> MVNISDFFGKNKKSVRSSTSRPTRQVGSSKPEVIDLDTESDQESTNKTPKKMPVSNVIDVSETPEGEKKLPLPAKRKASSPTVKPASSKKTKPSSKSSDSASNITAQDVLDKIPSLDLSNVHVKENAKFDFKSANSNADPDEIVSEIGSFPEGKPNCLLGLTIVFTGVLPTLERGASEALAKRYGARVTKSISSKTSVVVLGDEAGPKKLEKIKQLKIKAIDEEGFKQLIAGMPAEGGDGEAAEKARRKLEEQHNIATKEAELLVKKEEERSKKLAATRVSGGHLERDNVREEDKLWTVKYAPTNLQQVCGNKGSVMKLKNWLANWENSKKNSFKHAGKDGSGVFRAAMLYGPPGIGKTTAAHLVAQELGYDILEQNASDVRSKTLLNAGVKNALDNMSVVGYFKHNEEAQNLNGKHFVIIMDEVDGMSGGDRGGVGQLAQFCRKTSTPLILICNERNLPKMRPFDRVCLDIQFRRPDANSIKSRLMTIAIREKFKLDPNVIDRLIQTTRGDIRQVINLLSTISTTTKTINHENINEISKAWEKNIALKPFDIAHKMLDGQIYSDIGSRNFTLNDKIALYFDDFDFTPLMIQENYLSTRPSVLKPGQSHLEAVAEAANCISLGDIVEKKIRSSEQLWSLLPLHAVLSSVYPASKVAGHMAGRINFTAWLGQNSKSAKYYRLLQEIHYHTRLGTSTDKIGLRLDYLPTFRKRLLDPFLKQGADAISSVIEVMDDYYLTKEDWDSIMEFFVGPDVTTAIIKKIPATVKSGFTRKYNSMTHPVAIYRTGSTIGGGGVGTSTSTPDFEDVVDADDNPVPADDEETQDSSTDLKKDKLIKQKAKPTKRKTATSKPGGSKKRKTKA;> MSKTLSLQLPWVEKYRPQVLSDIVGNKETIDRLQQIAKDGNMPHMIISGMPGIGKTTSVHCLAHELLGRSYADGVLELNASDDRGIDVVRNQIKHFAQKKLHLPPGKHKIVILDEADSMTAGAQQALRRTMELYSNSTRFAFACNQSNKIIEPLQSRCAILRYSKLSDEDVLKRLLQIIKLEDVKYTNDGLEAIIFTAEGDMRQAINNLQSTVAGHGLVNADNVFKIVDSPHPLIVKKMLLASNLEDSIQILRTDLWKKGYSSIDIVTTSFRVTKNLAQVKESVRLEMIKEIGLTHMRILEGVGTYLQLASMLAKIHKLNNKA;> MSTSTEKRSKENLPWVEKYRPETLDEVYGQNEVITTVRKFVDEGKLPHLLFYGPPGTGKTSTIVALAREIYGKNYSNMVLELNASDDRGIDVVRNQIKDFASTRQIFSKGFKLIILDEADAMTNAAQNALRRVIERYTKNTRFCVLANYAHKLTPALLSRCTRFRFQPLPQEAIERRIANVLVHEKLKLSPNAEKALIELSNGDMRRVLNVLQSCKATLDNPDEDEISDDVIYECCGAPRPSDLKAVLKSILEDDWGTAHYTLNKVRSAKGLALIDLIEGIVKILEDYELQNEETRVHLLTKLADIEYSISKGGNDQIQGSAVIGAIKASFENETVKANV;> MFEGFGPNKKRKISKLAAEQSLAQQPWVEKYRPKNLDEVTAQDHAVTVLKKTLKSANLPHMLFYGPPGTGKTSTILALTKELYGPDLMKSRILELNASDERGISIVREKVKNFARLTVSKPSKHDLENYPCPPYKIIILDEADSMTADAQSALRRTMETYSGVTRFCLICNYVTRIIDPLASRCSKFRFKALDASNAIDRLRFISEQENVKCDDGVLERILDISAGDLRRGITLLQSASKGAQYLGDGKNITSTQVEELAGVVPHDILIEIVEKVKSGDFDEIKKYVNTFMKSGWSAASVVNQLHEYYITNDNFDTNFKNQISWLLFTTDSRLNNGTNEHIQLLNLLVKISQL;> MSLWVDKYRPKSLNALSHNEELTNFLKSLSDQPRDLPHLLLYGPNGTGKKTRCMALLESIFGPGVYRLKIDVRQFVTASNRKLELNVVSSPYHLEITPSDMGNNDRIVIQELLKEVAQMEQVDFQDSKDGLAHRYKCVIINEANSLTKDAQAALRRTMEKYSKNIRLIMVCDSMSPIIAPIKSRCLLIRCPAPSDSEISTILSDVVTNERIQLETKDILKRIAQASNGNLRVSLLMLESMALNNELALKSSSPIIKPDWIIVIHKLTRKIVKERSVNSLIECRAVLYDLLAHCIPANIILKELTFSLLDVETLNTTNKSSIIEYSSVFDERLSLGNKAIFHLEGFIAKVMCCLD;>[3x]GPHMASMLEAKFEEASLFKRIIDGFKDCVQLVNFQCKEDGIIAQAVDDSRVLLVSLEIGVEAFQEYRCDHPVTLGMDLTSLSKILRCGNNTDTLTLIADNTPDSIILLFEDTKKDRIAEYSLKLMDIDADFLKIEELQYDSTLSLPSSEFSKIVRDLSQLSDSINIMITKETIKFVADGDIGSGSVIIKPFVDMEHPETSIKLEMDQPVDLTFGAKYLLDIIKGSSLSDRVGIRLSSEAPALFQFDLKSGFLQFFLAPKFNDEE

Sliding clamps are ring-shaped protein complexes that are integral to the DNA replication machinery of all life. Sliding clamps are opened and installed onto DNA by clamp loader AAA+ ATPase complexes. The clamp loader of eukaryotes Replication Factor C (RFC) installs the sliding clamp Proliferating Cell Nuclear Antigen (PCNA) in a coordinated and stepwise fashion. In contrast to typical AAA+ ATPases, clamp loaders are heteropentameric with the five different subunits called A–E.

To reveal how RFC:PCNA binds and responds to DNA, we analyzed two classes that contain DNA-bound RFC:PCNA. One class shows PCNA in an open lock-washer shape, and the other has PCNA in a closed conformation. Therefore, we term these two states DNAPCNA-open and DNAPCNA-closed, respectively. Both classes contain clear density for p/t-DNA: 18 basepairs of duplex DNA are bound inside the central chambers of RFC and PCNA, and 6 nucleotides of the ssDNA template extend through the A-gate, preventing its closure. In DNAPCNA-open, both RFC and PCNA broadly resemble the conformations seen in Open1 and Open2. The RFC A-gate is open, with all five subunits gripping PCNA in an open lock-washer shape. However, both RFC and PCNA constrict relative to the Open1 and Open2 structures. PCNA constricts ~12 Å upon DNA binding, with most of this constriction occurring in subunit III of PCNA. Unexpectedly, we observe that the 3′ nucleotide of the primer strand is melted in both DNA-bound RFC:PCNA structures, with the base flipped away from the rest of the duplex. The DNAPCNA-open structure contains p/t-DNA and an open clamp, which is the transient intermediate following DNA binding.>[2x]MGDSDVPNDILEEQLYNSIVVADYDSAVEKSKHLYEEKKSEVITNVVNKLIRN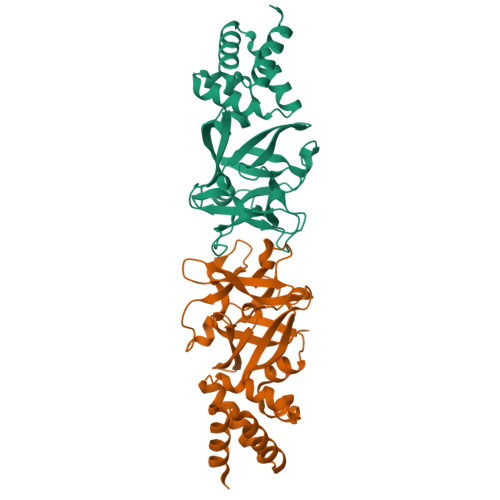NKMNCMEYAYQLWLQGSKDIVRDCFPVEFRLIFAENAIKLMYKRDGLALTLSNDVHGNDGRLAFGDGKDKTSPKVSWKFIALWENNKVYFKILNTERNQYLVLGVGTNPNGDHMAFGVNSVDSFRAQWYLQPAKYDKDNLFYIYNREYSKALTLSRTLETSGNRMAWGYNGRVIGSPEHYAWGVKAFAAALEHHHHHH> SNAMKRYRT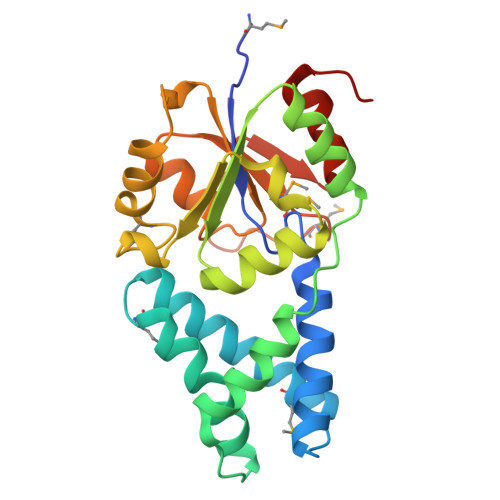LLFDVDDTILDFQAAEALALRLLFEDQNIPLTNDMKAQYKTINQGLWRAFEEGKMTRDEVVNTRFSALLKEYGYEADGALLEQKYRRFLEEGHQLIDGAFDLISNLQQQFDLYIVTNGVSHTQYKRLRDSGLFPFFKDIFVSEDTGFQKPMKEYFNYVFERIPQFSAEHTLIIGDSLTADIKGGQLAGLDTCWMNPDMKPNVPEIIPTYEIRKLEELYHILNIENTVSC> MYKNVPIWAQKWKPTIKALQSINVKDLKIDPSFLNIIPDDDLTKSVQDWVYATIYSIAPELRSFIELEMKFGVIIDAKGPDRVNPPVSSQCVFTELDAHLTPNIDASLFKELSKYIRGISEVTENTGKFSIIESQTRDSVYRVGLSTQRPRFLRMSTDIKTGRVGQFIEKRHVAQLLLYSPKDSYDVK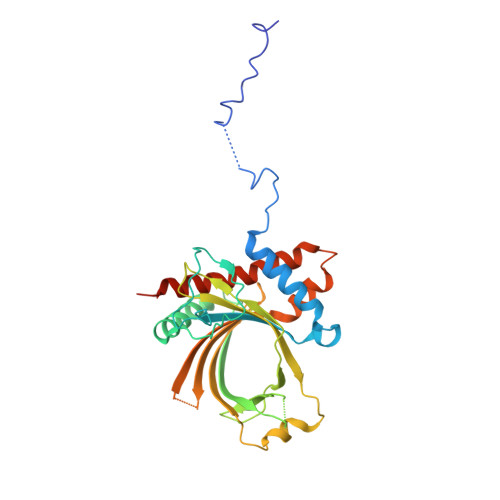ISLNLELPVPDNDPPEKYKSQSPISERTKDRVSYIHNDSCTRIDITKVENHNQNSKSRQSETTHEVELEINTPALLNAFDNITNDSKEYASLIRTFLNNGTIIRRKLSSLSYEIFEGSKKVM> KVFERCELARTLKRLGMDGYRGISLANWMCLAKWESGYNTRATNYNAGDRSTDYGI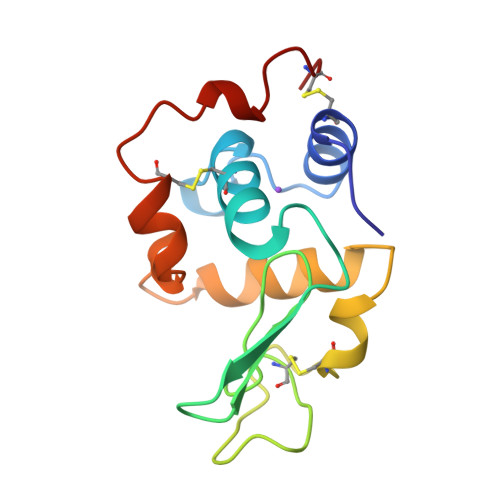FQINSRYWCNDGKTPGAVNAAHLSCSALLQDNIADAAAAAKRVVRDPQGIRAWVAWRNRCQNRDVRQYVQGCGV>MERAMEQLNRLTRSLRRARTVELPEDNETAVYTLMPMVMADQHRSVSELLSNSKFDVNYAFGRVKRSLLHIAANCGSVECLVLLLKKGANPNYQDISGCTPLHLAARNGQKKCMSKLLEYSADVNICNNEGLTAIHWLAVNGRTELLHDLVQHVSDVDVEDAMGQTALHVACQNGHKTTVQCLLDSGADINRPNVSGATPLYFACSHGQRDTAQILLLRGAKYLPDKNGVTPLDLCVQGGYGETCEVLIQYHPRLFQTIIQMTQNEDLRENMLRQVLEHLSQQSESQYLKILTSLAEVATTNGHKLLSLSSNYDAQMKSLLRIVRMFCHVFRIGPSSPSNGIDMGYNGNKTPRSQVFKPLELLWHSLDEWLVLIATELMKNKRDSTEITSILLKQKGQDQDAASIPPFEPPGPGSYENLSTGTRESKPDALAGRQEASADCQDVISMTANRLSAVIQAFYMCCSCQMPPGMTSPRFIEFVCKHDEVLKCFVNRNPKIIFDHFHFLLECPELMSRFMHIIKAQPFKDRCEWFYEHLHSGQPDSDMVHRPVNENDILLVHRDSIFRSSCEVVSKANCAKLKQGIAVRFHGEEGMGQGVVREWFDILSNEIVNPDYALFTQSADGTTFQPNSNSYVNPDHLNYFRFAGQILGLALNHRQLVNIYFTRSFYKHILGIPVNYQDVASIDPEYAKNLQWILDNDISDLGLELTFSVETDVFGAMEEVPLKPGGGSILVTQNNKAEYVQLVTELRMTRAIQPQINAFLQGFHMFIPPSLIQLFDEYELELLLSGMPEIDVSDWIKNTEYTSGYEREDPVIQWFWEVVEDITQEERVLLLQFVTGSSRVPHGGFANIMGGSGLQNFTIAAVPYTPNLLPTSSTCINMLKLPEYPSKEILKDRLLVALHCGSYGYTMA[2x]

HACE1 (HECT domain and Ankyrin repeat (AKR) containing E3 Ubiquitin Protein Ligase 1) is an AKR‐containing HECT E3 ligase in the “Other” subfamily. HACE1 is composed of an AKR domain at its N‐terminus (aa 26–252), a MID domain (aa 253–522) in the middle of the protein, and a HECT domain at its C‐terminus (aa 523–909). HACE1 is a tumor suppressor E3 ligase that has been reported to inhibit breast cancer cell proliferation through 26S proteasome‐mediated degradation of RAC1. Here, we report the cryo‐EM structures of monomeric and dimeric HACE1 along with in vitro biochemical assays.

Through 2D classification, we identified a G‐shaped HACE1 monomer and a circular dimer in which the subunits faced each other in an anti‐parallel orientation. Global resolution was 3.9 Å for the monomer and 4.6 Å for the dimer by gold standard FSC using a 0.143 cutoff. Our cryo‐EM structure shows that the HACE1 homodimer makes two head‐to‐tail contacts between the N‐terminal AKR domain of one monomer and the C‐terminal HECT domain of the other. The N‐terminal helix and the connecting loop dock into the groove of the small N‐lobe of the HECT domain. In the dimer, residues Arg13, Arg16, and Arg17 of one monomer interacts with Glu705, Tyr687, Glu712, and Thr707 of the other monomer. There are two interfaces present in the dimer which constituted 2421 and 2418 Å2 buried surface areas, respectively. In our HACE1 dimer, the N‐terminal helix and connective loop occupy the putative E2‐conjugating enzyme binding site of the other subunit. We hypothesize that obstruction of the small N‐lobe of the HECT domain could hinder the binding and activity of the E2‐conjugating enzyme, thereby modulating HACE1 enzymatic activity. Consistently, the HECT domain small N‐lobe of the dimer is slightly expanded compared with that of the monomer. Superimposition of the HECT domains of HACE1 monomer and dimer reveals the movement of the HECT domain C‐lobe by 17.2° which in turn causes the catalytic cysteine (C876) to slant by 14.7°.Some bacteriophage encode a recombinase that catalyzes single-stranded DNA annealing (SSA). Redβ belongs to a large group of proteins annotated as the RecT family based on the protein from the rac prophage of E. coli. Here, we have used single-particle cryo-EM to determine a 3.4 Å structure of a homolog of λ-Redβ from the A118 prophage of Listeria innocua that we will refer to as LiRecT. The structure confirms that the RecT/Redβ family of annealing proteins share a common core fold with RAD52.

Standard single-particle analysis without helical symmetry averaging in cryoSPARC yielded a 3.4 Å reconstruction with fully interpretable density for the LiRecT subunits and the bound DNA at the central portion of the filament. The filament has an open corkscrew-like shape with an inner diameter of 20 Å, an outer diameter of 100 Å, and a pitch of 105 Å with approximately 10 subunits per turn. The two complementary 83-mer strands are bound as a highly extended and un-wound duplex to a deep, narrow, positively-charged groove that runs along the outer surface of the filament. One strand, which we call “inner” and color in yellow is bound to the deepest part of the groove with its nucleotide bases facing outwards. The other strand, which we call “outer” (orange) is bound to the outer portion of the groove with its bases facing inward to form normal Watson-Crick base pairs with the inner strand. Each monomer of LiRecT binds to 5 bp of DNA. Consequently, we chose to refine a model that consists of just the 10 subunits of protein and 48 bp of DNA at the central portion of the filament, for which the density is strongest. Although most of the contacts involve the sugar-phosphate backbone of each strand, the side chains of V98, Y100, and Q107 from the β1–β2 hairpin wedge into the base pairs at every 5th bp step to separate them. Overall, the duplex is about 1.5 times as extended as B-form DNA and is completely unwound.

>GSHMATNDELKNQLANKQNGGQVASAQSLDLKGLLEAPTMRKKFEKVLDKKAPQFLTSLLNLYNGDDYLQKTDPMTVVTSAMVAATLDLPIDKNLGYAWIVPYKGRAQFQLGYKGYIQLALRTGQYKSINVIEVREGELLKWNRLTEEIELDLDNNTSEKVVGYCGYFQLINGFEKTVYWTRKEIEAHKQKFSKSDFGWKKDYDAMAKKTVLRNMLSKWGILSIDMQTAVTEDEAEPRERKDVTDDESIPDIIDAPVTPSDTLEAGSVVQGSMI[10x]> STDNAETGVIEAGNTDTDFSGELAAPGSNHTNVKFLFDRSRLLNVIKVLEKDAVFPRPFPTQEGAQQDDGYFCLLTPRPTVASRPATRFGLYANPSGSGVLANTSLDFNFYSLACFTYFRSDLEVTVVSLEPDLEFAVGWFPSGSEYQAS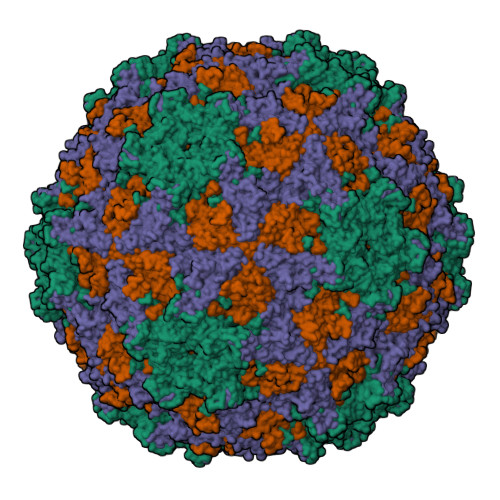SFVYDQLHVPFHFTGRTPRAFASKGGKVSFVLPWNSVSSVLPVRWGGASKLSSATRGLPAHADWGTIYAFVPRPNEKKSTAVKHVAVYIRYKNARAWCPSMLPFRSYKQKMLM;> GPIPTAPRENSLMFLSTLPDDTVPAYGNVRTPPVNYLPGEITDLLQLARIPTLMAFERVPEPVPASDTYVPYVAVPTQFDDRPLISFPITLSDPVYQNTLVGAISSNFANYRGCIQITLTFCGPMMARGKFLLSYSPPNGTQPQTLSEAMQCTYSIWDIGLNSSWTFVVPYISPSDYRETRAITNSVYSADGWFSLHKLTKITLPPDCPQSPCILFFASAGEDYTLRLPVDCNPSYVFH;> DHNTEEMENSADRVTTQTAGNTAINTQSSLGVLCAYVEDPTKSDPPSSSTDQPTTTFTAIDRWYTGRLNSWTKAVKTFSFQAVPLPGAFLSRQGGLNGGAFTATLHRHFLMKCGWQVQVQCNLTQFHQGALLVAMVPETTLDVKPDGKAKSLQELNEEQWVEMSDDYRTGKNMPFQSLGTYYRPPNWTWGPNFINPYQVTVFPHQILNARTSTSVDINVPYIGETPTQSSETQNSWTLLVMVLVPLDYKEGATTDPEITFSVRPTSPYFNGLRNRYTAGTDEEQ;> GNVQTTSKNDFDSRGNNGNMTFNYYANTYQNSVDFSTSSSASGAGPGNSRGGLAGLLTNFSGILNPLGYLK8-cyclopropyl-N-[5-methyl-1-(oxan-4-yl)-1H-pyrazol-4-yl]quinazolin-2-amine | C20 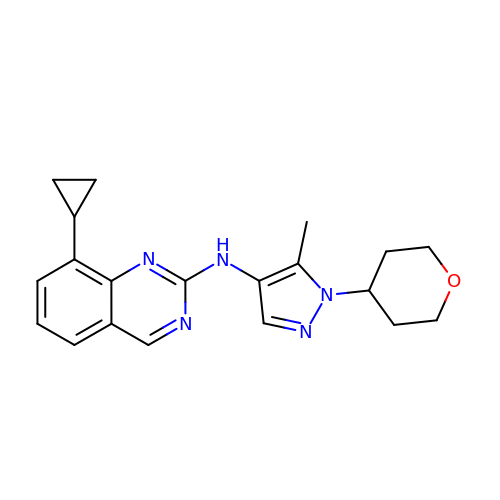H23 N5 O | FQSXQNNVERFAFF-UHFFFAOYSA-N>[4x]SNAMLIIETLPLLRQQIRRWRQEGKRIALVPTMGNLHEGHMTLVDEAKTRADVVVVTIFVNPLQFERPDDLAHYPRTLQEDCEKLTRHGADLVFAPAAADIYPAGL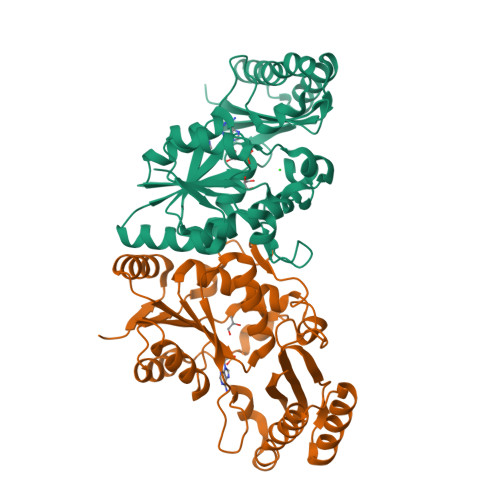EKQTYVDVPALSTILEGASRPGHFRGVSTIVSKLFNLIQPDVACFGEKDYQQLALIRKMVADMGYDINIVGVPTVRAKDGLALSSRNGYLTEEERQIAPQLSKIMWALAEKMALGERQIDALLEEAAAQLLRVGFTPDELFIRDAETLQPLTVDSQQAVILMAAWLGKARLIDNQLVDLRH> MSPQKRVKNVQAQNRTSQGSSSFQTTLSAWKVKQDPSNSKNISKHGQNNPVGDYEHADDQAEEDALQMAVGYFEKGPIKASQNKDKTLEKHLKTVENVAWKNGLASEEIDILLNIALSGKFGNAVNTRILKCMIPATVISEDSVVKAVSWLCVGKCSGSTKVLFYRWLVAMFDFIDRKEQINLLYGFFFASLQDDALCPYVCHLLYLLTKKENVKPFRVRKLLDLQAKMGMQPHLQALLSLYKFFAPALISVSLPVRKKIYFKNSENLWKTALLAVKQRNRGPSPEPLKLMLGPANVRPLKRKWNSLSVIPVLNSSSYTKECGKKEMSLSDCLNRSGSFPLEQLQSFPQLLQNIHCLELPSQMGSVLNNSLLLHYINCVRDEPVLLRFYYWLSQTLQEECIWYKVNNYEHGKEFTNFLDTIIRAECFLQEGFYSCEAFLYKSLPLWDGLCCRSQFLQLVSWIPFSSFSEVKPLLFDHLAQLFFTSTIYFKCSVLQSLKELLQNWLLWLSMDIHMKPVTNSPLETTLGGSMNSVSKLIHYVGWLSTTAMRLESNN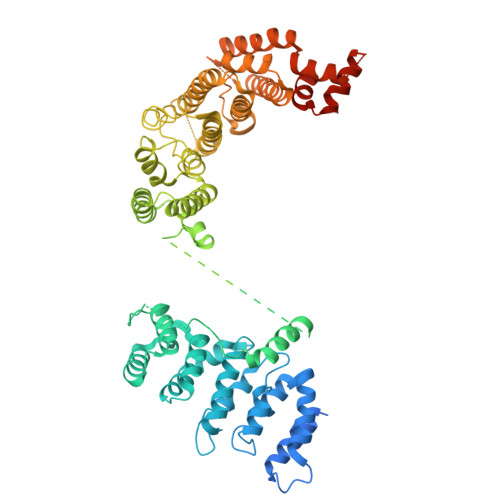TFLLHFILDFYEKVCDIYINYNLPLVVLFPPGIFYSALLSLDTSILNQLCFIMHRYRKNLTAAKKNELVQKTKSEFNFSSKTYQEFNHYLTSMVGCLWTSKPFGKGIYIDPEILEKTGVAEYKNSLNVVHHPSFLSYAVSFLLQESPEERTVNVSSIRGKKWSWYLDYLFSQGLQGLKLFIRSSVHHSSIPRAEGINCNNQY> MRCSCAFLDKSVFAAKRRVIVPIHPTPNFPAHFIKSAFTTDPLKEKQKARFSSGGEAMREVQDIPKNLEGERSRRDLASRGDTEFQALVEFIEGASYDQLISGRRFKKVYDVLSENDDMFIWLCHTAMSVLNPGDMRSRLIYNHLRILAESV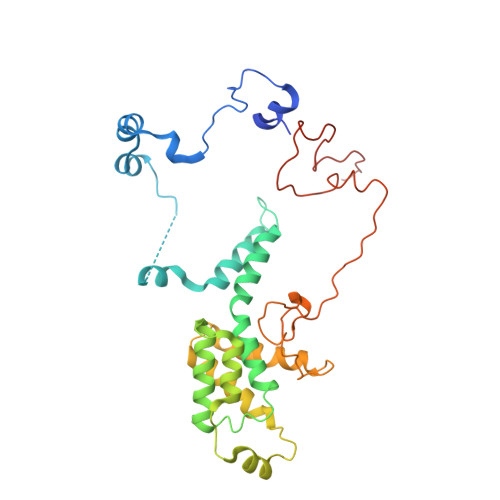ASGEMTQRTAFRFFESAVRSPAYREIAKRQLEGGAATRLAGISAAADVMRRMGLTRRPMSSYFELYQRIVERSEAMTPWGFPPLFQFEERLSLEPRLKFFSRASQQSLERRRRGHVMTPHTTLHGRRIFWIPPTWNRAGRFLGPHVTLYPGMTPD~{N}-[[1-[[3-[3,5-bis(chloranyl)phenyl]-5-[(4-piperidin-4-ylpiperidin-1-yl)methyl]phenyl]methyl]piperidin-4-yl]methyl]-2,2,2-tris(fluoranyl)ethanamide | C32 H41 Cl2 F3 N4 O | 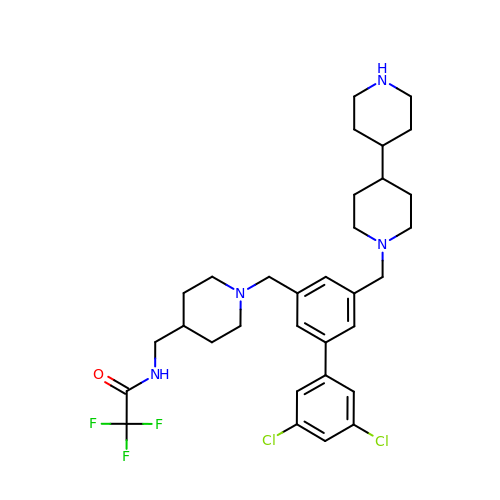OEDBVRNUMCXGJG-UHFFFAOYSA-N> DNSNNPVGGNPIDNYGTEHAPLLKEDNQYLVYQGERIVSFKDLLRRYQYLNSYWPQETGSGFRYYTLDSPGMPIYRGWDPNGIDQGQDSTAGNSPYNFCSMTLLNYLAPAFVCQRGSLRHKWVTAGARVNSTASVLSATRHGVLFPLPLAETAHPLDNALVGDRRSELQEMQRSRLNGTAITPVRLNNTLEIELPYYSIGQRFHASRFL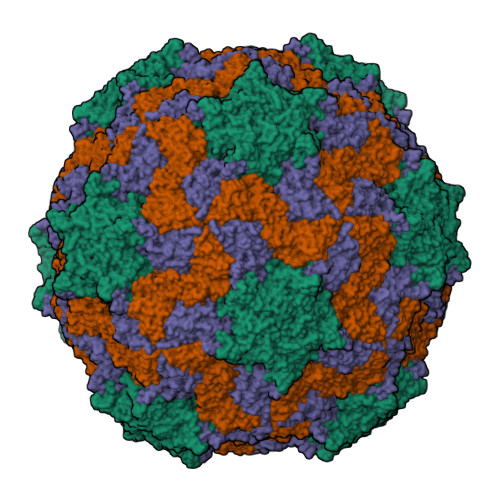DLAGTGDTQGVEIACEISDGGNDANYRLDQFVSVGEDFTLGMFVGAPIMYFYNDPTAT;> PSANDGPSFTTSKTSQNTTSENVHFVDGDTPWTYDVAATPDETSKLSGFDDAGLGEFLSRPIKIQQYQWTPGVQLFQTFNPWSDYFGNADVLEKINRFRNLRCKLCLKVLINGNSFYYGRALLSYNPYLRNDQVTVNRSFFIQDLIAASNKPHILLDPCSSEGGQMCLPFIWPENYLDITSTGWEDQMGECIIHDFDVLRHANGGTDPITVSIFAWAEDVSLLIPTTVAAQ;> SRPAVLSDIQPYVPRYCGNLANSDAPETVNKLSVDSKNELTIDTRTMGLGGADELTIHSIASRMTFWRQFDWPESAVTDTLLASMSVQPFCIDTVTASPVTEIHSTALAFASAPFETWQGSIKFHFKVVCSEYHRGRLRLVYNPLTNNAGPVAFNQVYSTTIDISNDREFDYECKWTDIRAWNACIGIDGATSATFFNTAAAVTGGTPFDNGTLSVYVVNELATPSTAAADVKVQVWVSAGDDFAVAVPGVGLSQLSYFQQQ;> EFKHDGLISKPASAVAKAADALSMIPYIAPYAKATSMVADKIGKIARIFGY7-{[3-(2-{[(6-aminopyridin-2-yl)methyl]amino}ethoxy)phenoxy]methyl}quinolin-2-amine | C24 H25 N5 O2 | 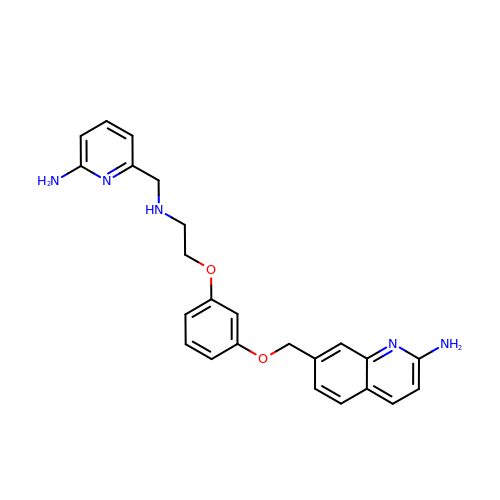ORKMBBJESKKJPF-UHFFFAOYSA-N>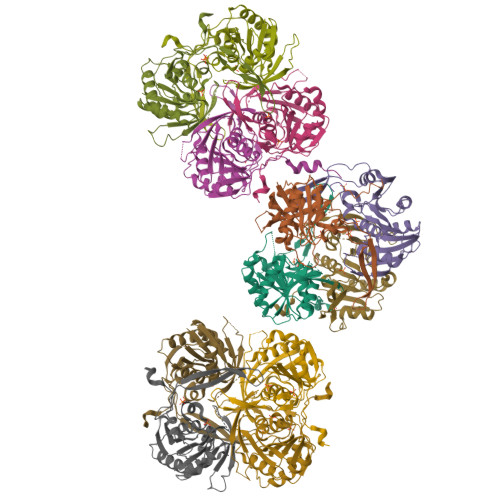[12x]MRILVTNDDGIYSPGLWALAEAASQFGEVFVAAPDTEQSAAGHAITIAHPVRAYPHPSPLHAPHFPAYRVRGTPADCVALGLHLFGPVDLVLSGVNLGSNLGHEIWHSGTVAAAKQGYLFGLSAAAFSVPLNGEVPDFAGLRPWLLRTLETLLRLERPFLVNVNLPLRPKGFLWTRQSVRAYEGVVIPGEDPMGRPFYWFAPRPLKEAEEGTDRWAVAQGFVSATPLRLDLTDETRLQPTLAHD Here we report on the galactomannan degradation machinery of the common human gut bacterium Bacteroides ovatus, with a focus on the extracellular, cell attached β-mannanase BoMan26B for which we here solve the crystal structure. As for other GH26 β-mannanases with determined structures, BoMan26B has a (β/α)8-barrel fold with an additional N-terminal α-helix and the two catalytic residues (predicted acid/base Glu-201 and nucleophile Glu-291 (50)) located in a cleft. Extracellular BoMan26B initially cleaves galactomannan into shorter oligosaccharides, which are transported into the periplasm by the SusC-like transporter.

To investigate the structural basis for the galactose side-group tolerance of BoMan26B, and the biochemical differences observed with BoMan26A, two crystal structures of BoMan26B were obtained: an apoenzyme structure and a structure containing the saccharide 63-α-d-galactosyl-mannotetraose (G1M4) in the active-site cleft. The two structures are very similar, 297 Cα atoms align with 0.148 Å root mean square deviation (RMSD), using PyMOL. A weak electron density was seen in the −1 and +1 subsites of the apoenzyme structure, but no molecule from expression, purification, or crystallization could be modeled with confidence. A calcium ion was modeled with 0.5 occupancy in the apoenzyme structure coordinated by Ser-108, Leu-105, and Glu-179 and three water molecules with a binding geometry typically seen for calcium. The calcium-binding site is not located in the active-site cleft and thus does not have a glycan-binding role. BoMan26B contains a potential calcium-binding site and was 100% stable over 24 h at 37 °C in the presence of 1 mm calcium, but it lost about 40% activity when it was not included. Trp-112 is situated in loop 2 that is also involved in the calcium-binding site. Thus, the calcium-binding site may play an important role in the correct conformation of the −5 subsite. A surface view of BoMan26A and BoMan26B reveals a more open active-site cleft in BoMan26B, with five subsites on the glycone side, whereas the BoMan26A cleft is narrower and restricted by loops 2 and 8, resulting in only two glycone-binding subsites. The longer and more open active-site cleft in BoMan26B correlates with its preference for longer substrates and production of a range of oligosaccharide products.

> MKNIYNFLIYFIFCGIGAGCSSSSGEDFPAPESEPVDNSLIKKELCTEGASVEAKKVYTYLRNCWGRKTLSSTMANVTWNVNEAIWVNRQTGKYPAIACFDYMNLPASPADWIDYNKISVVEDWWNAGGLVAACWHWNVPVTENSSEYKCMISETDFDITKALQEGTRENEIIKADLEELAGYLLLLKQKNIPVIWRPLHEAAGKWFWWGKDAASYKRLWKLVYETFKQKGLNNLIWVWTSETNDRDWYPGDAYVDIIGRDVYHKTSAAGLATDFDALKKAFPDKLIALSECGDVATIDKQLAAGAQWAWFMTWYDYEVTKDTTAPVFNSGQHEHADKAWWNNAFGQPGVICRSDLPSFKLEHHHHHH> MATALYTANDFILISLPQNAQPVTAPGSKTDSWFNETLIGGRAFVSDFKIPEFKIGSLDTLIVESEELSKVDNQIGASIGKIIEILQGLNETSTNAYRTLPINNMPVPEYLENFQWQTRKFKLDKSIKDLITLISNESSQLDADVRATYANYNSAKTNLAAAERKKTGDLSVRSLHDIVKPEDFVLNSEHLTTVLVAVPKSLKSDFEKSYETLSKNVVPASASVIAEDAEYVLFNVHLFKKNVQEFTTAAREKKFIPREFNYSEELIDQLKKEHDSAASLEQSLRVQLVRLAKTAYVDVFINWFHIKALRVYVESVLRYGLPPHFNIKIIAVPPKNLSKCKSELIDAFGFLGGNAFMKDKKGKIN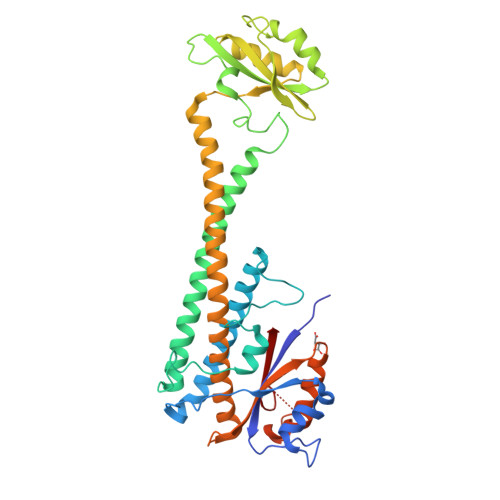KQDTSLHQYASLVDTEYEPFVMYIINL>MTTAPQEPPARPLQAGSGAGPAPGRAMRSTTLLALLALVLLYLVSGALVFRALEQPHEQQAQRELGEVREKFLRAHPCVSDQELGLLIKEVADALGGG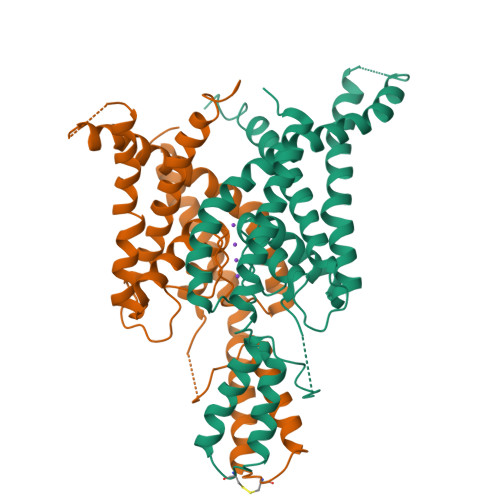ADPETQSTSQSSHSAWDLGSAFFFSGTIITTIGYGNVALRTDAGRLFCIFYALVGIPLFGILLAGVGDRLGSSLRHGIGHIEAIFLKWHVPPELVRVLSAMLFLLIGCLLFVLTPTFVFCYMEDWSKLEAIYFVIVTLTTVGFGDYVAGADPRQDSPAYQPLVWFWILLGLAYFASVLTTIGNWLRVVSRRTRAEMGGLTAQSNSLEVLFQ[2x]> MPISPIETVPVKLKPGMDGPKVKQWPLTEEKIKALVEICTEMEKEGKISKIGPENPYNTPVFAIKKKDSTKWRKLVDFRELNKRTQDFWEVQLGIPHPAGLKKKKSVTVLDVGDAYFSVPLDEDFRKYTAFTIPSINNETPGIRYQYNVLPQGWKGSPAIFQSSMTKILEPFRKQNPDIVIYQYMDDLYVGSDLEIGQHRTKIEELRQHLLRWGLTTPDKKHQKEPPFLWMGYELHPDKWTVQPIVLPEKDSWTVNDIQKLVGKLNWASQIYPGIKVRQLCKLLRGTKALTEVIPLTEEAELELAENREILKEPVHGVYYDPSKDLIAEIQKQGQGQWTYQIYQEPFKNLKTGKYARMRGAHTNDVKQLTEAVQKITTESIVIWGKTPKFKLPIQKETWETWWTEYWQATWIPEWEFVNTPPLVKLWYQLEKEPIVGAETFYVDGAANRETKLGKAGYVTNRGRQKVVTLTDTTNQKTELQAIYLALQDSGLEVNIVTDSQYALGIIQAQPDQSESELVNQIIEQLIKKEKVYLAWVPAHKGIGGNEQVDKLVSAGIRKVL;> MPISPI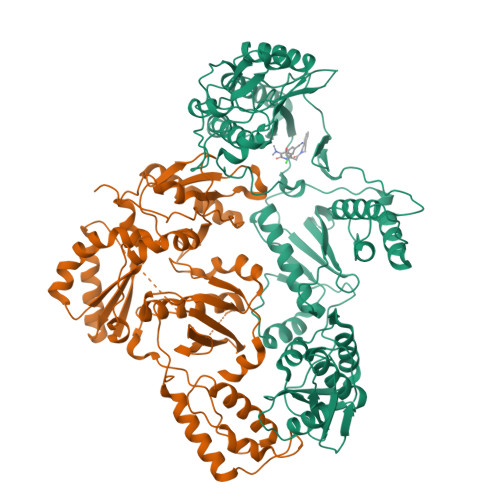ETVPVKLKPGMDGPKVKQWPLTEEKIKALVEICTEMEKEGKISKIGPENPYNTPVFAIKKKDSTKWRKLVDFRELNKRTQDFWEVQLGIPHPAGLKKKKSVTVLDVGDAYFSVPLDEDFRKYTAFTIPSINNETPGIRYQYNVLPQGWKGSPAIFQSSMTKILEPFRKQNPDIVIYQYMDDLYVGSDLEIGQHRTKIEELRQHLLRWGLTTPDKKHQKEPPFLWMGYELHPDKWTVQPIVLPEKDSWTVNDIQKLVGKLNWASQIYPGIKVRQLCKLLRGTKALTEVIPLTEEAELELAENREILKEPVHGVYYDPSKDLIAEIQKQGQGQWTYQIYQEPFKNLKTGKYARMRGAHTNDVKQLTEAVQKITTESIVIWGKTPKFKLPIQKETWETWWTEYWQATWIPEWEFVNTPPLVKLWYQLEKEPIVGAETF>MKVRVKAPCTSANLGVGFDVFGLCLKEPYDVIEVEAIDDKE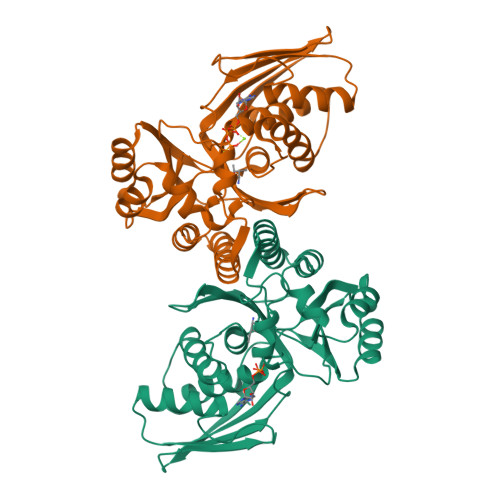IIIEVDDKNIPTDPDKNVAGIVAKKMIDDFNIGKGVKITIKKGVKAGSGLGSSAASSAGTAYAINELFKLNLDKLKLVDYASYGELASSGAKHADNVAPAIFGGFTMVTNYEPLEVLHIPIDFKLDILIAIPNISINTKEAREILPKAVGLKDLVNNVGKACGMVYALYNKDKSLFGRYMMSDKVIEPVRGKLIPNYFKIKEEVKDKVYGITISGSGPSIIAFPKEEFIDEVENILRDYYENTIRTEVGKGVEVV[4x]> 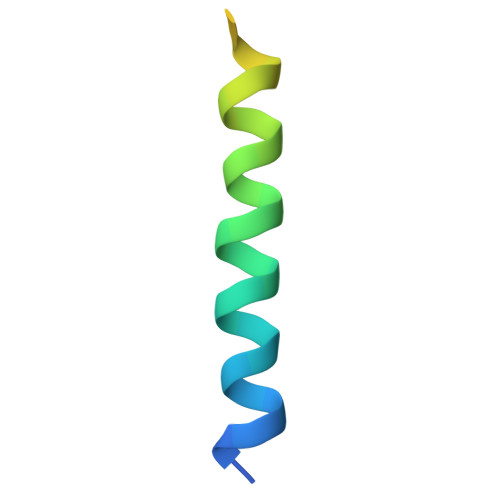SGSLDEAANYLYQSLLDDAVVGIFNETHHLRKSGNLAALDGV The enzymes are homotrimeric, with two cupredoxin-like domains in each monomer that harbour one type 1 copper (T1Cu) and one type 2 copper (T2Cu) site. The catalytic T2Cu site is located at the interface between two monomers, with a (His)3–H2O ligand coordination, while the T1Cu site is located near the surface of the protein. Two residues, Asp98 (AspCAT) and His255 (HisCAT) in Achromobacter cycloclastes CuNiR (AcNiR) numbering, that are conserved in all CuNiRs and are located either side of the T2Cu, are required for enzymatic activity. AspCAT is hydrogen-bonded to the copper H2O ligand and also to HisCAT via an H2O bridge.

The SF-ROXOX structure was compared with the 0.90 Å resolution synchrotron-radiation (SR) structure of AcNiR, revealing conservation of the overall structure with an all-protein-atom r.m.s.d. of 0.29 Å. The T2Cu is ligated by a single, highly ordered water molecule (W1) bound in a distorted tetrahedral geometry relative to the histidine plane. The active-pocket residues HisCAT and Ile257 (IleCAT) were in similar positions; however, there were marked differences in the positioning of the AspCAT residue and its hydrogen-bonding network. In the SF-ROXOX structure the proximal conformation of the AspCAT side chain has two variants of the proximal conformation compared with a single proximal conformation in the synchrotron structure. The additional conformation is formed by a 34° rotation around the Oδ1 atom, with the carboxyl Oδ2 atom forming a hydrogen bond to W1 at 3 Å, while the Oδ2 atom of the original conformation makes two hydrogen bonds to two water molecules, W3 and W4, one of which, W3, subsequently hydrogen-bonds to the T2Cu-ligated W1. In contrast, our SF-ROX structure of as-isolated AcNiR reported here shows that the T2Cu is ligated to a water molecule. It is the first time that this catalytically important water has been observed in a crystallographic structure obtained using femtosecond pulses from an X-ray laser. The distorted proximal position of AspCAT seen only in our SF-ROX structure shortens the hydrogen bond between the Oδ2 atom of Asp98 and the T2Cu water ligand W1 from 3.5 to 3 Å.

> MTEQLQMTRRTMLAGAALAGAVAPLLHTAQAHAAGAAAAAGAAPVDISTLPRVKVDLVKPPFVHAHDQVAKTGPRVVEFTMTIEEKKLVIDREGTEIHAMTFNGSVPGPLMVVHENDYVELRLINPDTNTLLHNIDFHAATGALGGGALTQVNPGEETTLRFKATKPGVFVYHCAPEGMVPWHVTSGMNGAIMVLPRDGLKDEKGQPLTYDKIYYVGEQDFYVPKDEAGNYKKYETPGEAYEDAVKAMRTLTPTHIVFNGAVGALTGDHALTAAVGERVLVVHSQANRDTRPHLIGGHGDYVWATGKFRNPPDLDQETWLIPGGTAGAAFYTFRQPGVYAYVNHNLIEAFELGAAGHFKVTGEWNDDLMTSVVKPASM> EMKPHPWFFGKIPRAKAEEMLSKQRHDGAFLIRESESAPGDFSLSVKFGNDVQHFKVLRDGAGKYFLG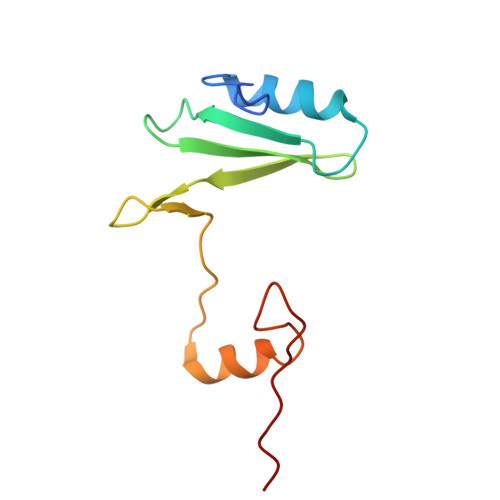VVKFNSLNELVDYHRSTSVSRNQQIFLRDIEQ> MIKKILIANRGEIAVRIVRACSEMGIKSVAIYSDADRHALH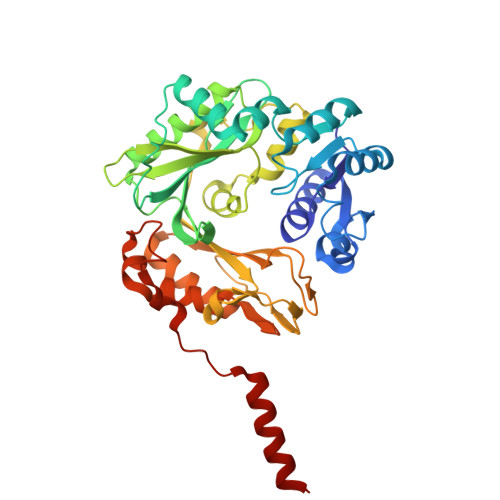VKKADEAYNIGSDPVLGYLNAHNIVNLAVASGCDALHPGYGFLSENPELAEICARRGIKFIGPDAKVIRQMGDKIQARTAMIKAGIPCVGSSGVVNPRHIEVQVLADSHGNVIHLFERDCSIQRRNQKLIEIAPSPQLSKAQREYIGNLAVKAAKAVGYKNAGTVEFLLDSDNNFYFMEMNTRLQVEHTVTEQITGIDIVQEQIRVADGQRLQYKQSEVQYRGFAMEFRINAEDPKNDFLPSFGKITRYYAPGGPGIRMDAAMYSGYVIPPYYDSMCAKLTVWALNWESVVERGRRALNDTVVYGVKTTIPYYQEILKHPDFRNAIFNTSFVESHPELANYATQFPRELVAAAISAAIAAHEGI> PGSMNELKHAVVPIDLQSFCLEGTLALWVPALENDSEDDSEAIETADDNEKLFKKECVAYDAGVYTSNKSKGSQTLRWSIFQNRTLTIFDVSLNSKKEPLSKFNVKIHFPSNVMKDGVAFSFSEHSDTTIIYAITHARVLYYIRLSKTWFQLPDARLDDDWCLCYRPISFLNQKPDLMAAISTSEICVSFFNGGLTKIILNPKDASHYEQHIDDSSYLFSLKKYLSLQAFKADYRSPNTIISMIFLSTYNVLVMLSLDYKLKVLDLSTNQCVETIELSQTILPLQSFPYLTSDHTTNSFIALYYPDNSHGSFSIYKLNANAHSFKLNVVIEKGIIPPSLPDDEFIPWMLSDFQLISSEGSQSKFLLIIAWKSNLNTVIQKCNLSLDQDESFSCVWSHSLDSFSLIEKTFFDVPTNMSSGDISEIWLQHIFAHNTSIESIQVALLSFQNSSSQVSKNKLDKFGALTISELKNAVLSSIVSTIQIEPNSDLTGYDYYEYKRLLYNEWERFAKLVAYLDHFGDEILSINFDPSNAVTYINYANKVAFIRDPYLIESFDEEPLTKLISSLETDDPSLIEGYQILDLGRSLHSCMSFSTLSEIRYSLRELVQDLPSYSLFDTLWVFYDKHIYPNVDPDYISTLIDTLVSLENPMRDIDSLIQRLRSFDIYNHSAQSPSLFLCASVARVLDSILKKFQVSIEGFIFLLSLITSQQDYELQSKFAGCDKLFLSLLEDWRLVSFLLENSALLLEKFEEEDVDSTNCNLNTMEALASVNTALQFFSALNYSECFSESQISPLHATVISSLSAIFIRDDTENDLVTELVEKLFLFKQYNACMQLIGWLNSDPIAVYLKALIYLKSKEAVKAVRCFKTTSLVLYSHTSQFAVLREFQEIAEKYHHQNLLSCYYLHLSKKLFEESAYID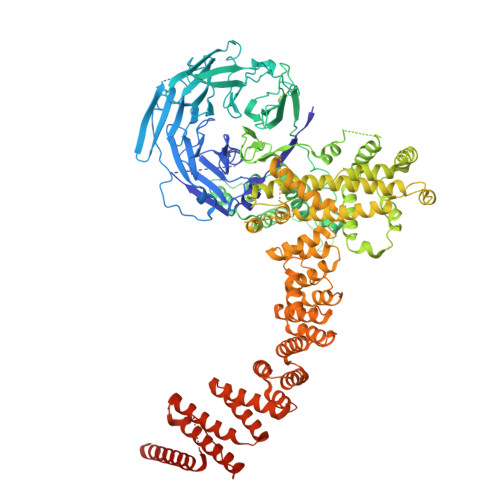ALEFSLLADASKETDDEDLSIAITHETLKTACAAGKFDAAHVALMVLSTTPLKKSCLLDFVNQLTKQGKINQLLNYSMPTLRQDVDNLLERKAFQMINVESQPCWYNILFSWRYKHQNYRDAAAIIYEKLSRYISTTELIGKKERTFIIEHYLIVLNTLELLPKEDTWILVTDMSVDKEPDPNFLPQKLLTLDAIVAEYHLQLKDVAVQVTAEMSSAMNIDL3'3'-cUMP-AMP | C19 H23 N7 O14 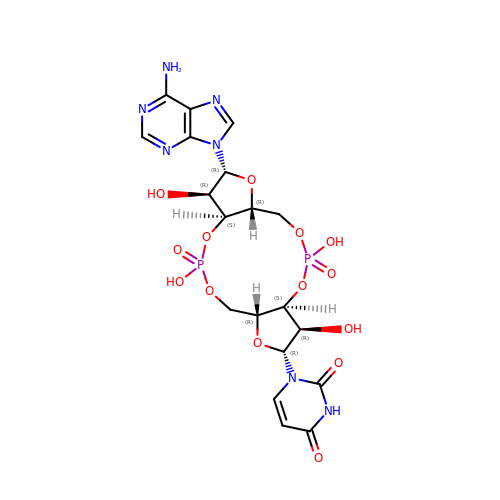P2 | CYVLWDUVMGUTIY-KPKSGTNCSA-N>[5x]MSLINTKIKPFKNQAFKNGEFIEITEKDTEGRWSVFFFYPADFTFVCPTELGDVADHYEELQKLGVDVYAVS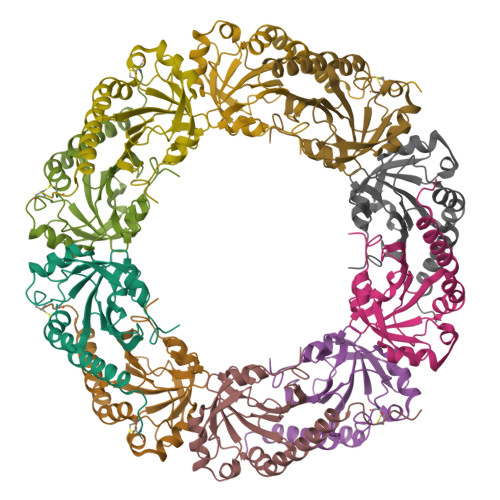TDTHFTHKAWHSSSETIAKIKYAMIGDPTGALTRNFDNMREDEGLADRATFVVDPQGIIQAIEVTAEGIGRDASDLLRKIKAAQYVASHPGEVCPAKWKE> MSSLAFRTLRNGLGLKSSVRALSTTTTTLSNYQQPDYSSYLNNKSGQGSRNFTYFMVGSMGLLSAAGAKSTVEAFLSSFAASADVLAMAKVEVKLGAIPEGKNVIIKWQGKPVFIRHRTA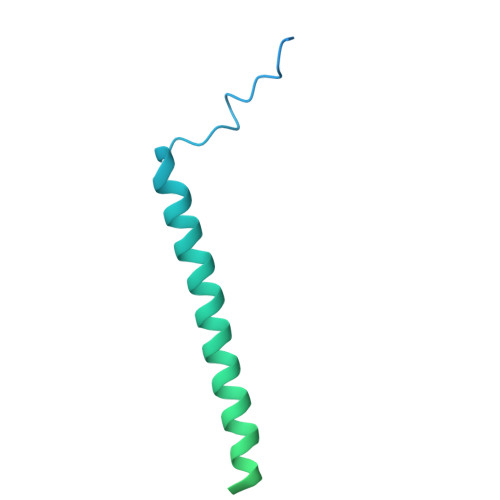DEIEEANQVDIKTLRDPQNDADRVKKPEWLIMLGICTHLGCVPIGEAGDFGGWFCPCHGSHYDISGRIRKGPAPLNLEIPEYDFTDDETLLVG> ANKLDSKKLTRSNGTTLEYS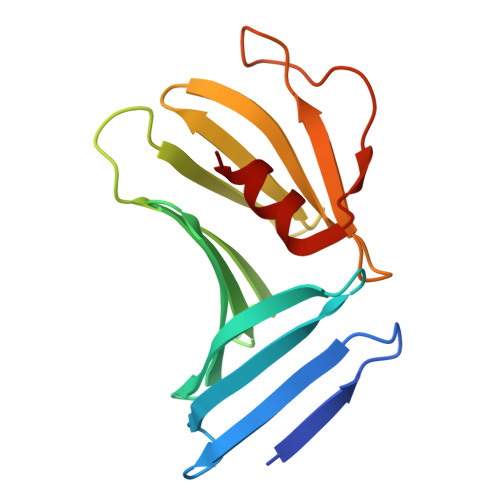QITDADNATKAVETLKNSIKLEGSLVVGKTTVEIKEGTVTLKREIEKDGKVKVFLNDTAGSNKKTGKWEDSTSTLTISADSKKTKDLVFLTDGTITVQQYNTAGTSLEGSASEIKNLSELKNALK4-AMINOPYRIDINE | C5 H7 N2 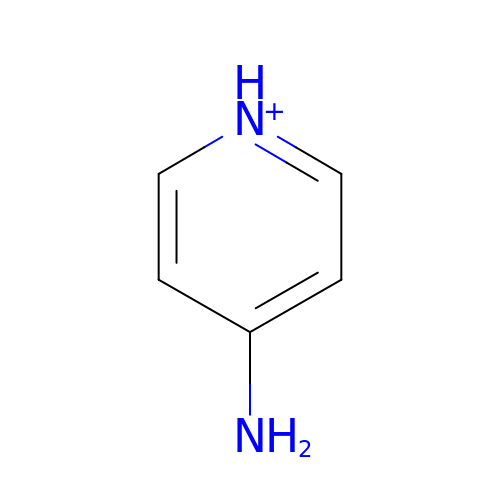| NUKYPUAOHBNCPY-UHFFFAOYSA-O> GSHMPEPTVEDVISQVARAHREIFTYAHDKLGSSPGNFNANHASGSPHGRSGRTVQEIWEDFSMSFTPAVREVVEFAKHIPGFRDLSQHDQVTLLKAGTFEVLMVRFAS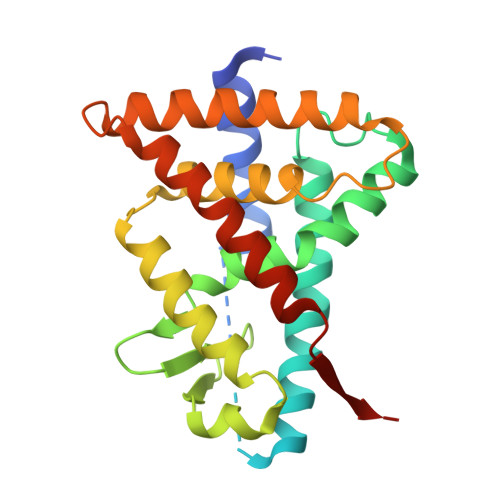LFNVKDQTVMFLSRTTYSLQELGAMGMGDLLSAMFDFSEKLNSLALTEEELGLFTAVVLVSADRSGMENSASVEQLQETLLRALRALVLKNRPLETSRFTKLLLKLPDLRTLNNMHSEKLLSFRVDAQ>TFGTFQDAYLSQLRDIYHSPEFRNAPRGQASRERIGAGFRLLDPVQRHISVPARRANVVFNFAEALWYLSGSDRLDFIQYYAPGIAAYSADGRTLRGTAYGPRIFRHPAGGVNQWENVVKTLTDDPDSKRAVIQIFDPRELAVADNIDVACTLALQFLIRDGLLCGIGYMRANDAFRGAVSDVFSFTFLQEFTARYLGLGIGTYHHVVGSVHIYDSDARWAERVLDAATPDGGPRPGFPAMPDGDNWPHVRRVLEWEERLRTNAARLSADALDALDLPAYWKHVVALFEAHRQVRHEDTPDRALLAALPEVYRQSLAVKWPGHFG[2x]

We previously demonstrated that MilA, a CMP hydroxymethylase in the mildiomycin biosynthetic gene cluster in Streptomyces rimofaciens ZJU5119, can convert CMP to hmCMP12. MilA and CH are akin to the superfamily of thymidylate synthases (TS), which transfers a methyl group from CH2THF to dUMP to form dTMP in the de novo thymidylate synthesis pathway and, hence, DNA synthesis. In this study, we demonstrated that MilA has a substrate preference for CMP (kcat/KM = 39.2 mM−1 min−1) over dCMP (kcat/KM = 7.84 mM−1 min−1), and thus offers an opportunity to investigate the mechanism by which conserved TS evolves the preference for ribosyl over 2′-deoxyribosyl groups. In the structures of apo MilA and its complexes with various substrates, MilA are all homodimers.

Subsequently, the structures of MilA‒CMP, MilA‒dCMP and MilA‒hmCMP complexes were refined to 1.65 Å, 2.10 Å and 1.80 Å resolution, respectively. The electron density for residues 305–308 was poor in the structure of apo MilA but resolved clearly in the structures of all the MilA‒substrate complexes.>[2x]KFSKEQLRTFQMIHENFGRALSTYLSGRLRTFVDVEISIDQLTYEEFIRSVMIPSFIVIFTGDVFEGSAIFEMRLDLFYTMLDIIMGGPGENPPNRPPTEIETSIMRKEVTNMLTLLAQAWSDFQYFIPSIENVETNPQFVQIVPPNEIVLLVTAS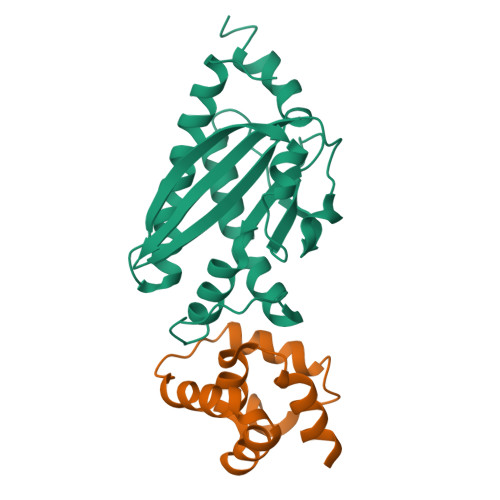VSWGEFTSFINVCWPFSLLEPLLEKLSDRFWM;>GSHMVQLVNFLQSEHPQTIAVVLSYLDPPVAAQILGALPEELQTEVLKRIALLERTSPEVVKEIERNLEKKISGFSRTFS[2x]> QVGVIKPWLLLGSQDAAHDLDTLKKNKVTHI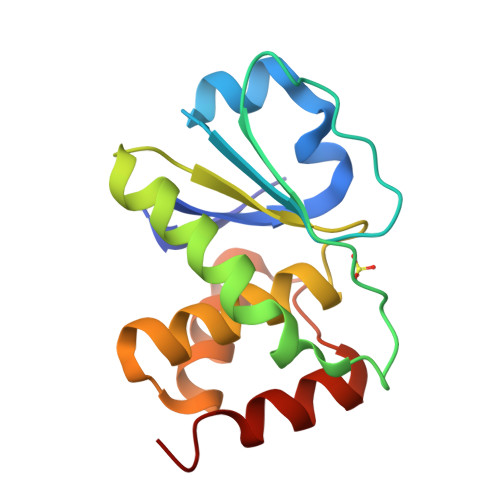LNVAYGVENAFLSDFTYKSISILDLPETNILSYFPECFEFIEEAKRKDGVVLVHSNAGVSRAAAIVIGFLMNSEQTSFTSAFSLVKNARPSACPNSGFMEQLRTYQEGK> METYIKLDKLGEGTYATVYKGKSKLTDNLVALKEIRLEHEEGAPCTAIREVSLLKDLKHANIVTLHDIIHTEKSLTLVFEYLDKDLKQYLDDCGNIINMHNVKLFLFQLLRGLAYCHRQKVLHRDLKPQNLLINERGELKLADFGLARAKSIPTKTYDNEVVTLWYRPPDILLGSTDYSTQIDMWGVGCIFYEMATGRPLFPGSTVEEQLHFIFRILGTPTEETWPGILSNEEFKTYNYPKY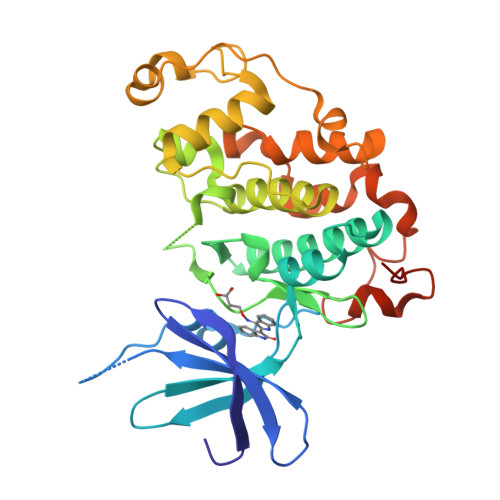RAEALLSHAPRLDSDGADLLTKLLQFEGRNRISAEDAMKHPFFLSLGERIHKLPDTTSIFALKEIQLQKEASLRSAHHHHHH>MGHHHHHHSSGLVPRGSHATAIVTNVKHFGGMGSALRLSEAGHTVACHDESFKQKDELEAFAETYPQLKPMSEQEPAELIEAVTSAYGQVDVLVSNDIFAPEFQPIDKYAVEDYRGAVEALQIRPFALVNAVASQMKKRKSGHIIFIT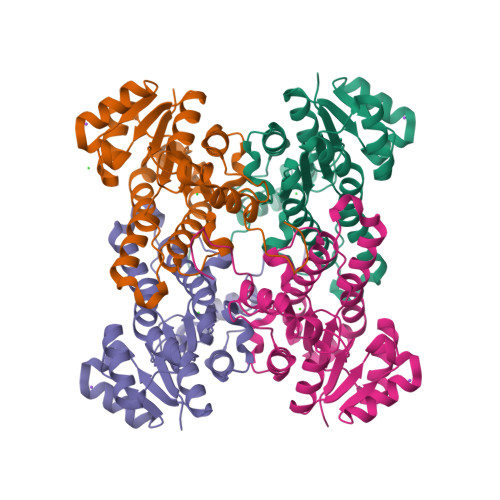SATPFGPWKELSTYTSARAGANTLANALSKELGEYNIPVFAIGPNYLHSEDSPYFYPTEPWKTNPEHVAHVKKVTALQRLGTQKELGELVAFLASGSCDYLTGQVFWLAGGFPMIERWPGMPE[4x]> MAEIVLDRVTKSYPDGAGGVRAAVKEFSMTIADGEFIILVGPSGCGKSTTLNMIAGLEEITSGELRIGGERVNEKAPKDRDIAMVFQSYALYPHMTVRQNIAFPLTLAKVPKAEIAAKVEETAKILDLSELLDRKPGQLSGGQRQRVAMGRAIVRSPKAFLMDEPLSNLDAKLRVQMRAEISRLQDRLGTTTVYVTHDQTEAMTLGDRVVVMLAGEVQQIGTPDELYSSPANLFVAGFIGSPAMNFFPATRTDVGVRLPFGEVTLTPHMLDLLDKQARPENIIVGIRPE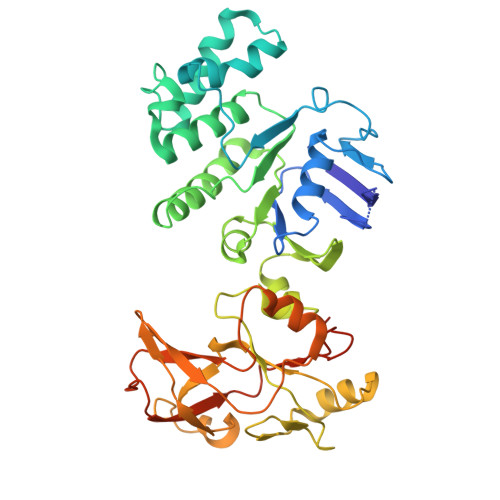HIEDSALLDGYARIRALTFSVRADIVESLGADKYVHFTTEGAGAESAQLAELAADSGAGTNQFIARVSADSRVRTGEQIELAIDTTKLSIFDAATGLNLTRDITPTDPTEAAGPDAG>[2x]MSHSLREWLAFLEGKGKLKRVRKEVDPVFEIAALGKQADGICSLLFERVKGYAVPVVTGLAGDRELFAAAMSVPVEGMLEKLAAAVENPVPCRLVSPDGAPVKECIIRENIDLLKMLPIPTHHAGDAGPYITAAILIARDPDSGV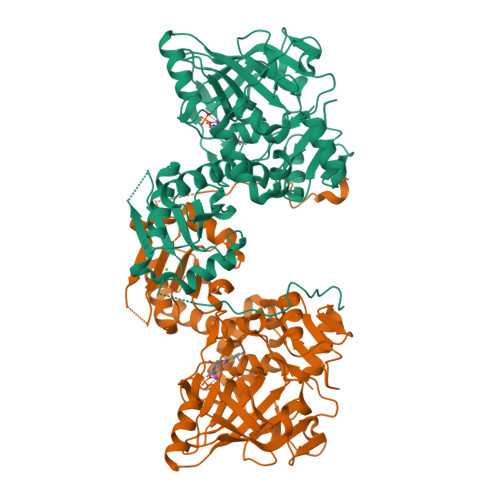RNVSIHRLQVTGPDRLGILILPRHLWHFFGKAERAGRPLEIALAIGVHPAVLLASQATTRLGVDELEIASALLPQPLELVKCETVDVEVPAGAEIVIEGKILPGVREVEGPFGEYPRYYGPAAPRPVVEVTAVTHRRQPVYHTIIPASREHLLLGGIAREAVLLQTVRQNVPTVKNVHLTPGGSCRYHAVISIEKKHEGEAKRAIDAAFNSSSEVKHVVVVDHEINIFDPEEVEWAVATRCQPGRDVTIFKDARGNRLDPSSRDGVSDKMGIDATIPLNLPGERFERISIPGLDKIKLADYLE>[4x]MGAVFKL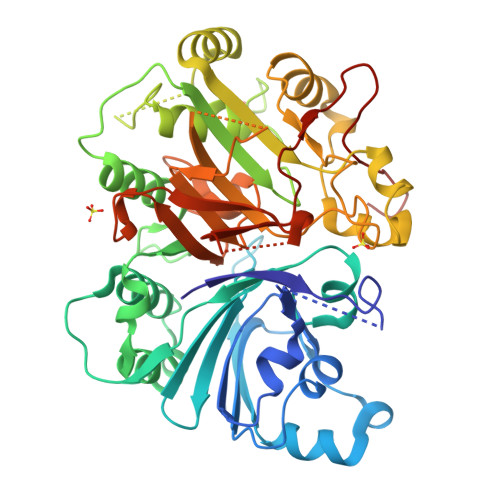MKSDFYEREDFMGEVEDMITLKDIFGTETLKRSILFSFQYELDFLLRQFHQNVENITIVGQKGTIMPIEARAMDATLAVILKKVKLIEITMPPFASHHTKLIINFYDNGECKIFLPSNNFTSMETNLPQQVCWCSPLLKIGKEGLPVPFKRSLIEYLNSYHLKDIDELITKSVEEVNFAPLSELEFVYSTPSKFQSSGLLSFYNKLEKLSAGTSASDTAKHYLCQTSSIGTSLSRARDENLWTHLMIPLFTGIMSPPAKDTAGRKKAEILPTNSLINEYSQRKIKPYIIFPTEQEFVTSPLKWSSSGWFHFQYLQKKSYYEMLRNKFKVFYKQDPAMVTRRRGTTPANSKFYMHCATNSAGPCDASQVFKELEWCLYTSANLSQTAWGTVSRKPRNYEAGVLYHSRRLANTRKVTCRTFTRDRRGCAGNPTHVAVPFTLPVIPYDLAEDECFCLALEHHHHHH> MAGVEEVAASGSHLNGDLDPDDREEGAASTAEEAAKKKRRKKKKSKGPSAAGEQEPDKESGASVDEVARQLERSALEDKERDEDDEDGDGDGDGATGKKKKKKKKKRGPKVQTDPPSVPICDLYPNGVFPKGQECEYPPTQDGRTAAWRTTSEEKKALDQASEEIWNDFREAAEAHRQVRKYVMSWIKPGMTMIEICEKLEDCSRKLIKENGLNAGLAFPTGCSLNNCAAHYTPNAGDTTVLQYDDICKIDFGTHISGRIIDCAFTVTFNPKYDTLLKAVKDATNTGIKCAGIDVRLCD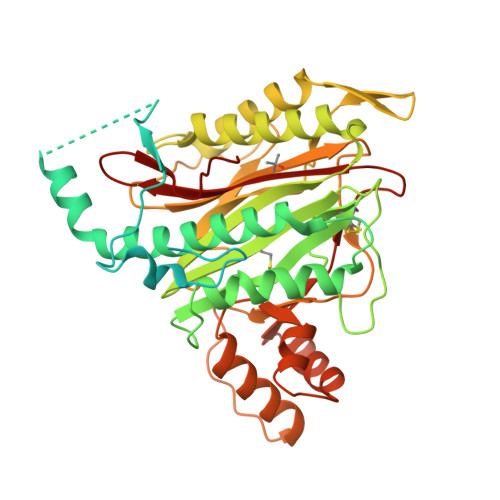VGEAIQEVMESYEVEIDGKTYQVKPIRNLNGHSIGQYRIHAGKTVPIIKGGEATRMEEGEVYAIETFGSTGKGVVHDDMECSHYMKNFDVGHVPIRLPRTKHLLNVINENFGTLAFCRRWLDRLGESKYLMALKNLCDLGIVDPYPPLCDIKGSYTAQFEHTILLRPTCKEVVSRGDDY>TWGVSSPKNVQGLSGSCLLIPCIFSYPADVPVSNGITAIWYYDYSGKRQVVIHSGDPKLVDKRFRGRAELMGNMDHKVCNL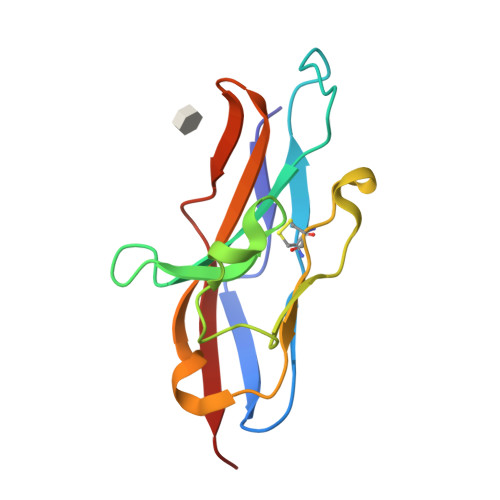LLKDLKPEDSGTYNFRFEISDSNRWLDVKGTTVTVTTD[2x]>[2x]MEILRYLMDPDTFTSNFNNDPLVLR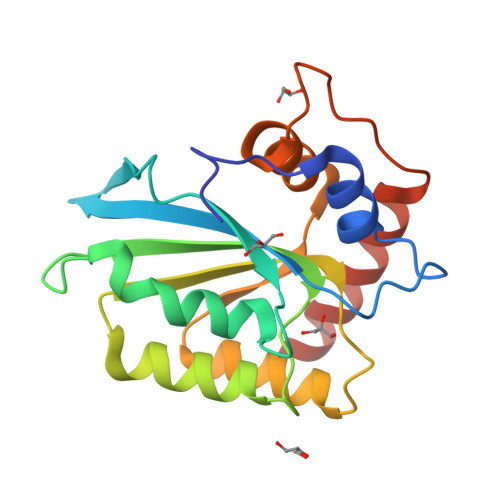RRQTYLCYEVERLDNGTSVKMDQHMGFLCNESGRHAELRFLDLVPSLQLDPAQIYRVTWFISWSPCFSWGCAGEVRAFLQENTHVRLRIKAARIYDYDPLYKEALQMLRDAGAQVSIMTYDEFEYCWDTFVYRQGCPFQPWDGLEEHSQALSGRLRAILQL>[2x]MKEVVIASAVRTAIGSYGKSLKDVPAVDLGATAIKEAVKKAGIKPEDVNEVILGNVLQAGLGQNPARQASFKAGLPVEIPAMTINKVCGSGLRTVSLAAQIIKAGDADVIIAGGMENMSRAPYLANNARWGYRMGNAKFVDEMITDGLWDAFNDYHMGITAENIAERWNISREEQDEFALASQKKAEEAIKSGQFKDEIVPVVIKGRKGETVVDTDEHPRFGSTIEGLAKLKPAFKKDGTVTAGNASGL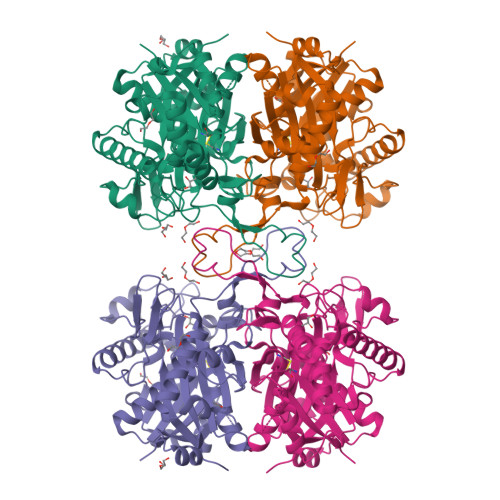NDCAAVLVIMSAEKAKELGVKPLAKIVSYGSAGVDPAIMGYGPFYATKAAIEKAGWTVDELDLIESNEAFAAQSLAVAKDLKFDMNKVNVNGGAIALGHPIGASGARILVTLVHAMQKRDAKKGLATLCIGGGQGTAILLEKCLEHHHHHH> HGYVASPGSRAFFGSSAGGNLNTNVGRAQWEPQSIEAPKNTFITGKLASAGVSGFEPLDEQTATRWHKTNITTGPLDITWN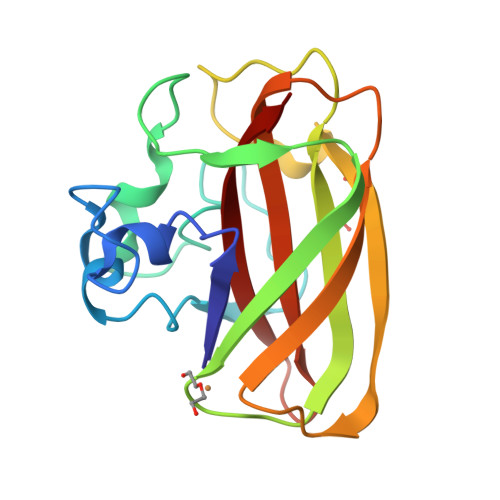LTAQHRTASWDYYITKNGWNPNQPLDIKNFDKIASIDGKQEVPNKVVKQTINIPTDRKGYHVIYAVWGIGDTVNAFYQAIDVNIQ>MRGSHHHHHHIQESRLDRILESGVLRVATTGDYKPFSYRTEEGGYAGFDVDMAQRLAESLGAKLVVVPTSWPNLMRDFADDRFDIAMSGISINLERQRQAYFSIPYLRDGKTPITLCSEEARFQTLEQIDQPGVTAIVNPGGTNEKFARANLKKARILVHPDNVTIFQQIVDGKADLMMTDAI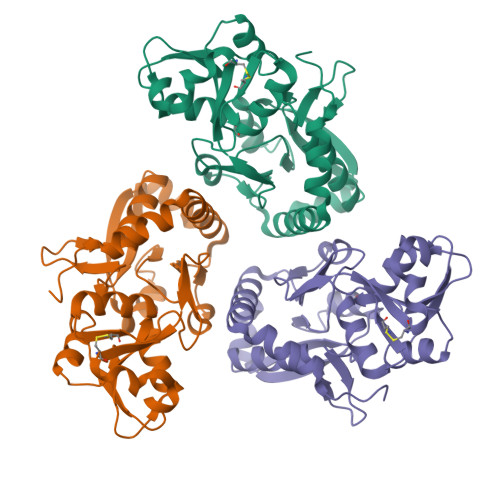EARLQSRLHPELCAVHPQQPFDFAEKAYLLPRDEAFKRYVDQWLHIAEQSGLLRQRMEHWLEYRWPTAHGKL[3x]> MSYQVLARKWRPQTFADVVGQEHVLTALANGLSLGRIHHAYLFSGTRGVGKTSIA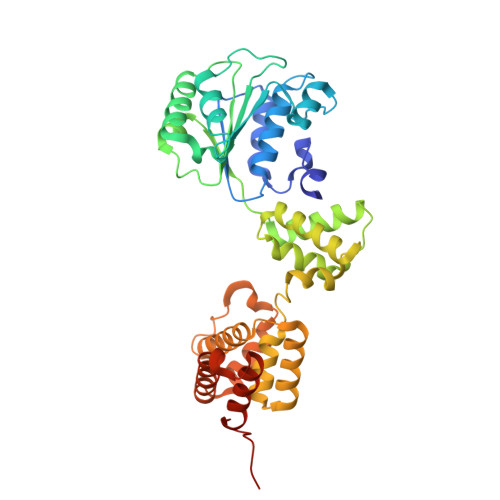RLLAKGLNCETGITATPCGVCDNCREIEQGRFVDLIEIDAASRTKVEDTRDLLDNVQYAPARGRFKVYLIDEVHMLSRHSFNALLKTLEEPPEHVKFLLATTDPQKLPVTILSRCLQFHLKALDVEQIRHQLEHILNEEHIAHEPRALQLLARAAEGSLRDALSLTDQAIASGDGQVSTQAVSAMLGTLDDDQALSLVEAMVEANGERVMALINEAAARGIEWEALLVEMLGLLHRIAMVQLSPAALGNDMAAIELRMRELARTIPPTDIQLYYQTLLIGRKELPYAPDRRMGVEMTLLRALAFHPRMPLPEPEVPRQ> MGKSAVIFVERATPATLTELKDALSNSILSVRDPWSIDFRTYRCSIKNLPADVSKLMYSITFHHHGRQTVLIKDNSAMVTTAAAADIPPALVFNGSSTGVPESIDTILSSKLSNIWMQRQLIKGDAGETLILDGLTVRLVNLFSSTGFKGLLIELQADEAGEFETKIAGIEGHLAEIRAKEYKTSSDSLGPD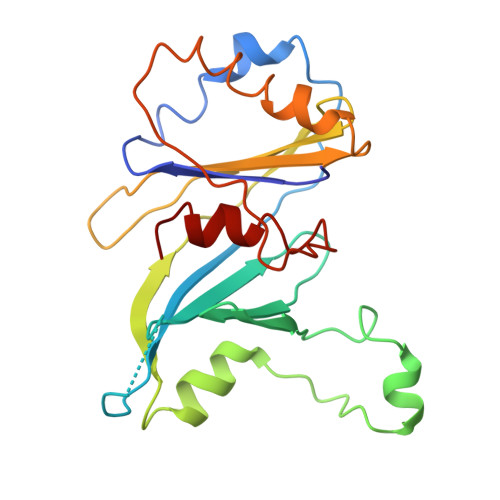TSNEICDLAYQYVRALEL> DDYSVVEEHGQLSISNGELVNERGEQVQLKGMSSHGLQWYGQFVNYESMKWLRDDWGINVFRAAMYTSSGGYIDDPSVKEKVKEAVEAAIDLDIYVIIDWHILSDNDPNIYKEEAKDFFDEMSELYGDYPNVIYEIANEPNGSDVTWGN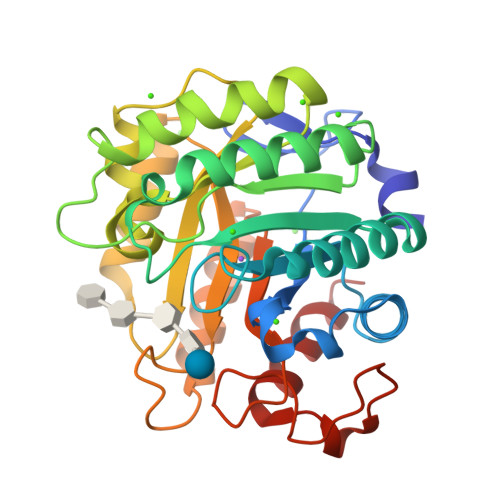QIKPYAEEVIPIIRNNDPNNIIIVGTGTWSQDVHHAADNQLADPNVMYAFHFYAGTHGQNLRDQVDYALDQGAAIFVSEWGTSAATGDGGVFLDEAQVWIDFMDERNLSWANWSLTHKDESSAALMPGANPTGGWTEAELSPSGTFVREKIRESA> LECHNQQSSQPPTTKTCPGETNCYKKVWRDHRGT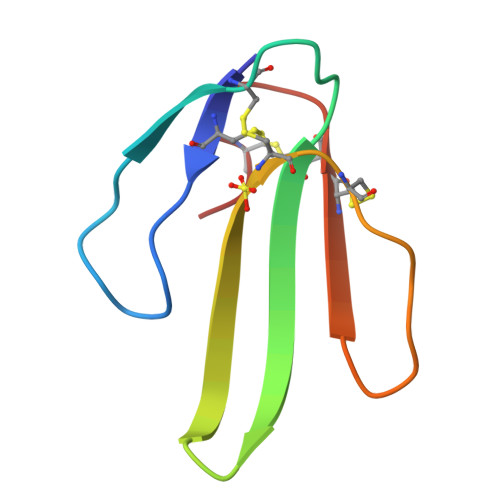IIERGCGCPTVKPGIKLNCCTTDKCNN>[4x]MKITAARVIITCPGRNFVTLKIETDQGVYGIGDATLNGRELSVVA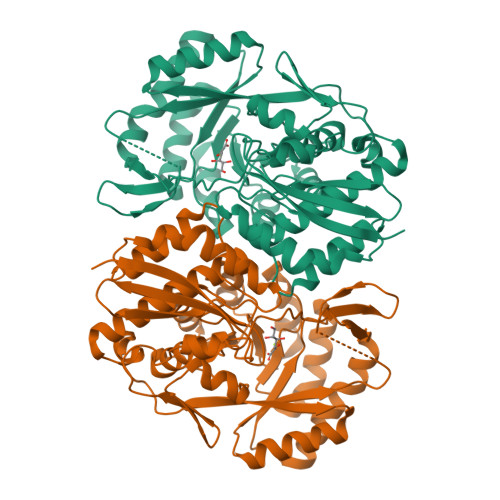YLQEHVAPCLIGMDPRRIEDIWQYVYRGAYWRRGPVTMRAIAAVDMALWDIKAKMAGMPLYQLLGGRSRDGIMVYGHANGSDIAETVEAVGHYIDMGYKAIRAQTGVPGIKDAYGVGRGKLYYEPADASLPSVTGWDTRKALNYVPKLFEELRKTYGFDHHLLHDGHHRYTPQEAANLGKMLEPYQLFWLEDCTPAENQEAFRLVRQHTVTPLAVGEIFNTIWDAKDLIQNQLIDYIRATVVGAGGLTHLRRIADLASLYQVRTGCHGATDLSPVTMGCALHFDTWVPNFGIQEYMRHTEETDAVFPHDYWFEKGELFVGETPGHGVDIDEELAAKYPYKPAYLPVARLEDGTMWNW>MAKPQVTILATGGTIAGSGESSVKSSYSAGAVTVDKLLAAVPAINDLATIKGEQISSIGSQEMTGKVWLKLAKRVNELLAQKETEAVIITHGTDTMEETAFFLNLTVKSQKPVVLVGAMRSGSSMSADGPMNLYNAVNVAINKASTNKGVVIVMNDEIHAAREATKLNTTAVNAFASPNTGKIGTVYYGKVEYFTQSVRPHTLASEFDISKIEELPRVDILYAHPDDTDVLVNAALQAGAKGIIHAGMGNGNPFPLTQNALEKAAKSGVVVARSSRVGSGSTTQEAEVDDKKLGFVATESLNPQKARVLLMLALTKTSDREAIQK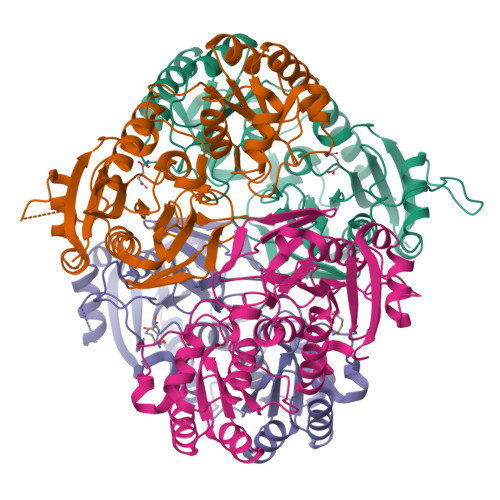IFSTY[8x]(2R,3R)-8-CYCLOPROPYL-7-(NAPHTHALEN-1-YLMETHYL)-5-OXO-2-PHENYL-2,3-DIHYDRO-5H-[1,3]THIAZOLO[3,2-A]PYRIDINE-3-CARBOXYLIC ACID | C28 H23 N O3 S | 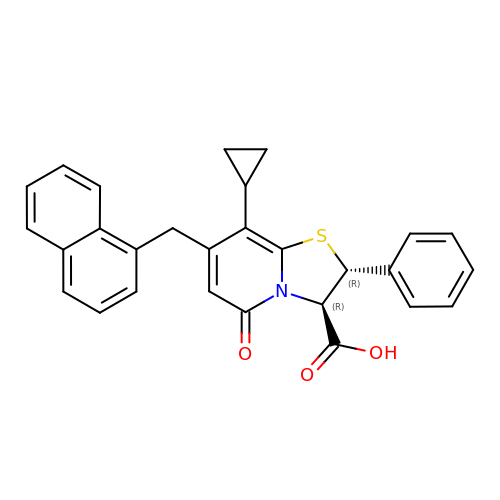QSGWJHVTILGJTA-IZZNHLLZSA-N> MGRMLTIRVFKYDPQSAVSKPHFQEYKIEEAPSMTIFIVLNMIRETYDPDLNFDFVCRAGICGSCGMMINGRPSLACRTLTKDFED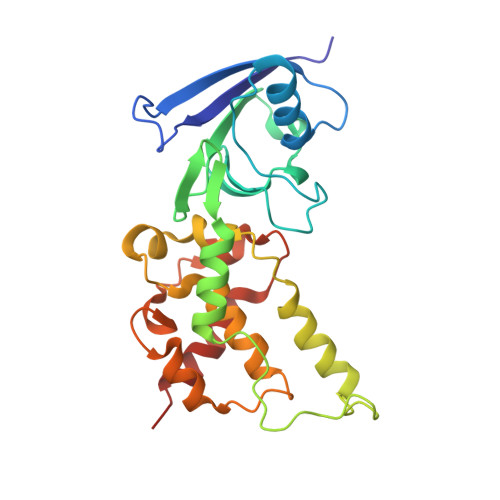GVITLLPLPAFKLIKDLSVDTGNWFNGMSQRVESWIHAQKEHDISKLEERIEPEVAQEVFELDRCIECGCCIAACGTKIMREDFVGAAGLNRVVRFMIDPHDERTDEDYYELIGDDDGVFGCMTLLACHDVCPKNLPLQSKIAYLRRKMVSVNMS> GDVTFDVGDEYEIIETIGNGAYGVVSSARRRLTGQQVAIKKIPNAFDVVTNAKRTLRELKILKHFKHDNIIAIKDILRPTVPYGEFKSVYVVLDLMESDLHQIIHSSQPLTLEHVRYFLYQLLRGLKYMHSAQVIHRDLKPSNLLVNENCELKIGDFGMARGLCTSPAEHQYFMTEYVATRWYRAPELMLSLHEYTQAIDLWSVGCIFGEMLARRQLFPGKNYVHQLQLIMMVLGTPSPAVIQAVGAERVRAYIQSLPPRQPVPWETVYPGADRQALSLLGRMLRFEPSARISAAAALRHPFLAKYHDPDDEPDCAPPFDFAFDREALTRERIKEAIVAEIEDFHARREGIRQQIRFQ

Extracellular signal-regulated kinase 5 (ERK5) is a member of the mitogen-activated protein kinase (MAPK) family, which includes ERK1/2, JNK1/2/3, and p38. Activation of the nonclassical MEK5–ERK5 MAPK pathway is associated with increased cellular proliferation, migration, survival, and angiogenesis. In approximately 50% of hepatocellular carcinomas (HCCs), the MAPK7 gene encoding for ERK5 is amplified. Phosphorylated ERK5 associates with, phosphorylates, and activates a number of downstream transcription factors, such as the myocyte enhancer factor (MEF) family, c-Myc, RSK, c-Fos, c-Jun, and Sap1a,8 which are involved in the modulation of apoptosis. Selective ERK5 kinase inhibitors will therefore be useful in elucidating the role of this signaling protein in cancer and determining whether they represent potential therapeutics.

Smaller, nonbasic analogue 34b provided the best balance of potency and in vitro ADME properties and had good oral bioavailability in mouse. However, N-methylpyrazole 34b had good permeability and low efflux and was also stable in mouse liver microsomes. The structure of 34b bound to ERK5 was solved to a resolution of 2.75 Å, confirming that the binding mode was maintained, with the pyrrole carboxamide forming a bidentate interaction with the hinge region of the ATP-binding site. The methylpyrrole amide lies in a small channel at the mouth of the binding pocket, lying between the side chain of E146 and the backbone of M140 and the lipophilic side chain on I61. The halogenated phenyl ring adopts a conformation orthogonal to the plane of the pyrrole ketone. Pyrazole amide 34b had low clearance and an oral bioavailability of 42% in the mouse. No inhibition or the closely related kinases ERK1 and ERK2 and JNKs 1, 2, and 3 were observed in a kinase panel screen, and 34b had an IC50 > 20 μM against BRD4, in contrast to some of the earlier reported ERK5 inhibitors. Thus, 34b represents a structurally distinct ERK5 inhibitor chemotype, which is a useful addition to the toolkit for interrogating ERK5 signaling. When examining a truncated ERK5 construct that lacked both the NLS and TAD (ERK5 ΔTAD), 34b inhibited its kinase activity in cells with an IC50 of 77 ± 4 nM (mean ± SEM, n = 5). However, a greater than 13-fold reduction in activity was observed (i.e., IC50 > 1 μM) when 34b was examined against full-length ERK5, suggesting that this compound also induces a paradoxical activation of ERK5 transcriptional activity.>GSHMTPDIILQRTGIDVRAVEQGDDAWHKLRLGVITASEVHNVIAKPRSGKKWPDMKMSYFHTLLAEVCTGVAPEVNAKALAWGKQYENDARTLFEFTSGVNVTESPIIYRDESMRTACSPDGLCSDGNGLELACPFTSRDFMKFRLGGFEAIKSAYMAQVQYSMWVTRKNAWYFANYDPRMKREGLHYVVIERDEKYM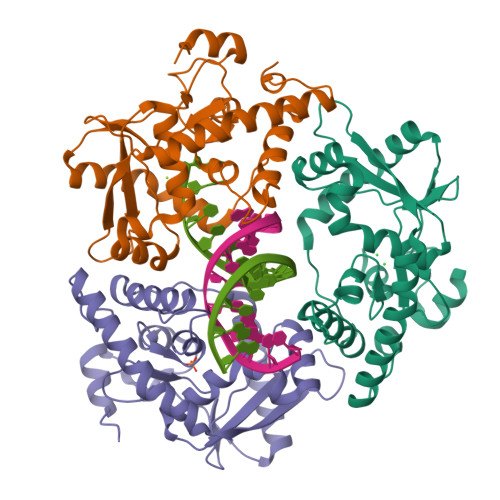ASFDEIVPEFIEKMDEALAEIGFVFGEQWR[3x]>MMFLRQEDFATVVRSTPLVSLDFIVENSRGEFLLGKRTNRPAQGYWFVPGGRVQKDETLEAAFERLTMAELGLRLPITAGQFYGVWQHFYDDNFSGTDFTTHYVVLGFRFRV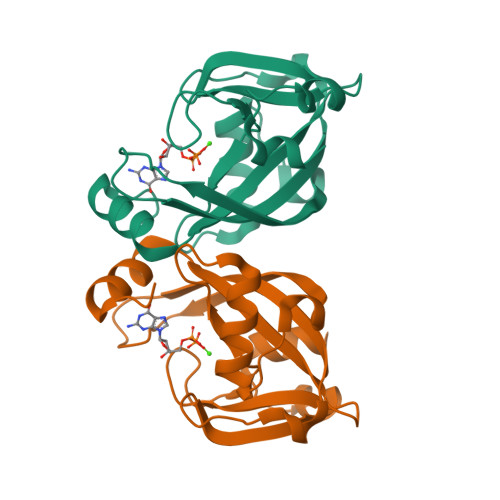AEEELLLPDEQHDDYRWLTPDALLASENVHANSRVYFNNDPRAIIGLNKKEVKNV[2x]>MDHAPERFDATPPAGEPDRPALGVLELTSIARGITVADAALKRAPSLLLMSRPVSSGKHLLMMRGQVAEVEESMIAAREIAGAGSGALLDELELPYAHEQLWRFLDAPVVADAWEEDTESVIIVETATVCAAIDSADAALKTAPVVLRDMRLAIGIAGKAFFTLTGELADVEAAAEVVRERCGARLLELACIARPVDELRGRLFF[3x];>[36x]MADALGMIEVRGFVGMVEAADAMVKAAKVELIGYEKTGGGYVTAVVRGDVAAVKAATEAGQRAAERVGE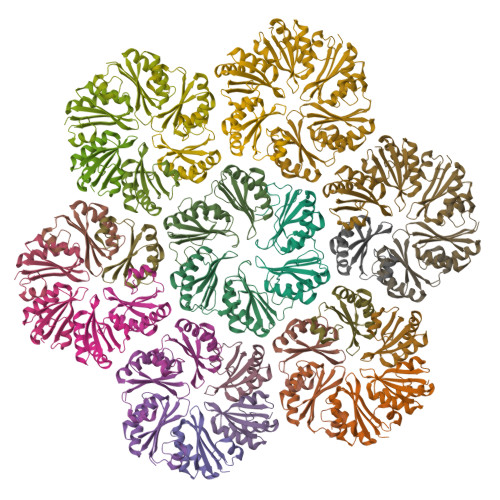VVAVHVIPRPHVNVDAALPLGRTPGMDKSA{(3S)-1-[5-(cyclohexylcarbamoyl)-6-(propylsulfanyl)pyridin-2-yl]piperidin-3-yl}acetic acid | C22 H33 N3 O3 S | 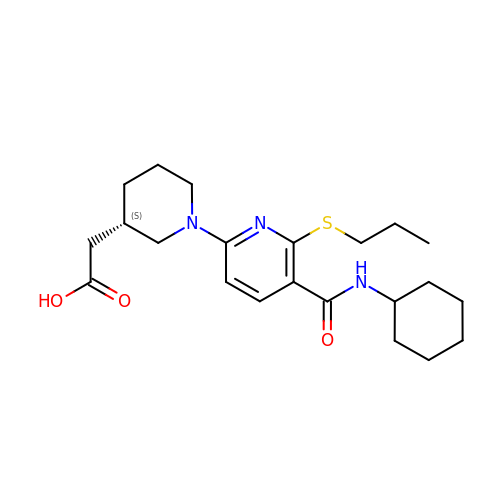NCDZABJPWMBMIQ-INIZCTEOSA-N> MAAVTLHLRAETKPLEARAALTPTTVKKLIAKGFKIYVEDSPQSTFNINEYRQAGAIIVPAGSWKTAPRDRIIIGLKEMPETDTFPLVHEHIQFAHC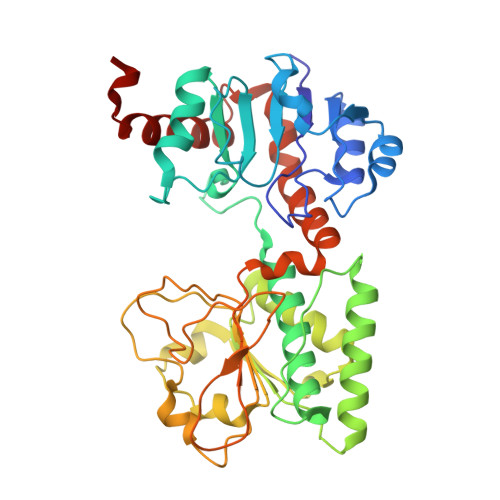YKDQAGWQNVLMRFIKGHGTLYDLEFLENDQGRRVAAFGFYAGFAGAALGVRDWAFKQTHSDDEDLPAVSPYPNEKALVKDVTKDYKEALATGARKPTVLIIGALGRSGSGAIDLLHKVGIPDANILKWDIKETSRGGPFDEIPQADIFINCIYLSKPIAPFTNMEKLNNPNRRLRTVVDVSADTTNPHNPIPIYTVATVFNKPTVLVPTTAGPKLSVISIDHLPSLLPREASEFFSHDLLPSLELLPQRKTAPVWVRAKKLFDRHCARVKRSSRL>[2x]HMEGPAGYLRRASVAQLTQELGTAFFQQQQLPAAMADTFLEHLCLLDIDSQPVAARSTSIIATIGPASRSVDRLKEMIKAGMNIARLNFSHGSHEYHAESIANIREATESFATSPLSYRPVAIALDTKGPEIRTGVLQGGPESEVEIVKGSQVLVTVDPKFQTRGDAKTVWVDYHNITRVVAVGGRIYIDDGL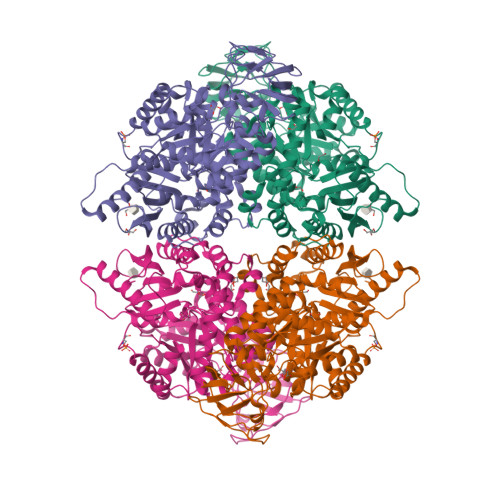ISLVVQKIGPEGLVTEVEHGGILGSRKGVNLPNTEVDLPGLSEQDLLDLRFGVQHNVDIIFASFVRKASDVLAVRDALGPEGQNIKIISKIENHEGVKKFDEILEVSDGIMVARGDLGIEIPAEKVFLAQKMMIGRCNLAGKPVVCATQMLESMITKARPTRAETSDVANAVLDGADCIMLSGETAKGSFPVEAVMMQHAIAREAEAAVYHRQLFEELRRAAPLSRDPTEVTAIGAVEASFKCCAAAIIVLTKTGRSAQLLSQYRPRAAVIAVTRSAQAARQVHLSRGVFPLLYREPPEAIWADDVDRRVQFGIESGKLRGFLRVGDLVIVVTGWRPGSGYTNIMRVLSVSHHHHHH> MEHAEHGNSNAPMEYQSETGRLNILGFWIFLGAEIVLFSTLFATFFVLKNRTAGGVLPDELFEVNLVMIMTFLLLISSFTCGIAVHEMRRGSLKGVVIWTIITLLLGAGFVGCEINEFVHYVHEGAALSTSAFWSGFFVLLGTHGTHVTIGIFWITGILIQLKKRGLTPQTSSKIFISSLYWHFLDVVWIF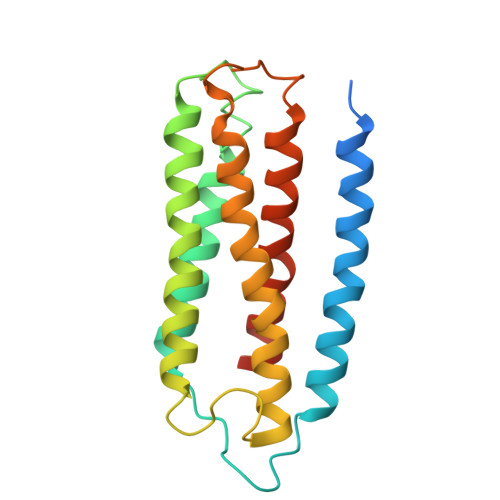IFTGVYLMGLGGL Human SNM1B (SNM1B, Apollo, or DCLRE1B) is a 5′-to-3′ exonuclease, which was first identified as one of three vertebrate orthologues of the yeast DNA repair nuclease, PSO2 (4). SNM1B is a member of the metallo-β-lactamase (MBL) structural superfamily, of which the β-CASP (CPSF, Artemis, SNM1, PSO2) nucleic acid processing nucleases are a subfamily. All MBL type enzymes possess a characteristic α/β/β/α MBL core fold that provides a scaffold that supports the active site, which coordinates the metal ions essential for catalysis. The SNM1B sequence comprises 532 amino acids, wherein the N-terminal region (amino acids 1–332) contains the catalytic (MBL and β-CASP) domains, and the C-terminal region the protein-protein interaction regions, including the well-characterised TRF2 binding domain (amino acids 498–509).

In addition to the structure of SNM1B1–355 (nucleotide form) we solved a structure of unliganded SNM1B1–355 to 2.8 Å resolution, hereafter denoted SNM1B1–355 (apo form). For the apo form, only the M1 metal binding site was occupied; XRF revealed iron, nickel, and zinc present in the crystal, with nickel being the most abundant. This metal ion is coordinated in an approximately octahedral conformation, with a bonding network (H31, H33, H99, D120, and a water molecule) and co-ordination distances in the region of 2.3 Å consistent with each Ni2+, Zn2+, Fe2+ (39). D35 which forms part of the second metal ion coordination site (M2) adopts a different sidechain conformation in the apo-structure compared to the nucleotide-form structure. Overlays of the structures of SNM1B1–355 (apo form) and SNM1B1–355 (nucleotide form) reveal they have the same architecture with similar relative domain orientations. The most prominent differences lie in the ordering of the extended loop connecting the final β-strand on the MBL domain with the C-terminal helix (residues 297–315), and smaller but still substantial shifts in the two regions connecting the MBL and β-CASP domains (residues 146–159 and 266–279). These regions cluster around the 5′-phosphate binding pocket, with significant shifts to both main chain and side chains required to accommodate the AMP_1 in the apo form structure, suggesting an induced pocket. Presumably, these regions are relatively flexible and move to form favourable interactions with DNA upon substrate binding. However, whether these structures represent the catalytically or physiologically relevant forms of SNM1B is not clear, and it is likely that the presence of Ni in both the apo and nucleotide form crystals is due to the use of Ni-Sepharose in the purification process.

> MNGVLIPHTPIAVDFWSLRRAGTARLFFLSHMHSDHTVGLSSTWARPLYCSPITAHLLHRHLQVSKQWIQALEVGESHVLPLDEIGQETMTVTLLDANHCPGSVMFLFEGYFGTILYTGDFRYTPSMLKEPALTLGKQIHTLYLDNTNCNPALVLPSRQEAAHQIVQLIRKHPQHNIKIGLYSLGKESLLEQLALEFQTWVVLSPRRLELVQLLGLADVFTVEEKAGRIHAVDHMEICHSNMLRWNQTHPTIAILPTSRKIHSSHPDIHVIPYSDHSSYSELRAFVAALKPCQVVPIVSRRPCGGFQDSLSPRISVPLIPDSVQQYMSSSSRKPSAENLYFQ>MAAFVVSTPKKLQTDELATVRLFQENTPSVVYITNLAVRQDAFTLDVLEVPQGSGSGFVWDKQGHIVTNYHVIRGASDLRVTLADQTTFDAKVVGFDQDKDVAVLRIDAPKNKLRPIPVGVSADLLVGQKVFAIGNPFGLDHTLTTGVISGLRREISSAATGRPIQDVIQTDAAINPGNSGGPLLDSSGTLIGINTAIYSPSGASSGVGFSIPVDTVGGIVDQLVRFGKVTRPILGIKFAPDQSVEQLGVSGVLVLDAPPSGPAGKAGLQSTKRDGYGRLVLGDIITSVNGTKVSNGSDLYRILDQCKVGDEVTVEV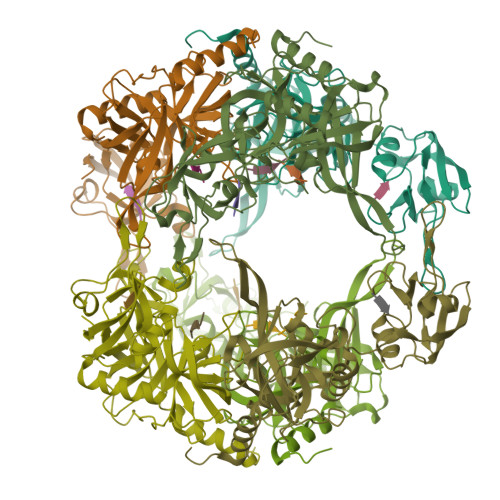LRGDHKEKISVTLEPKPDESAAALEHHHHHH[3x]> GGUUAAGUUAGGUUUGUGGUUGAAAGUCGAUGCCAGUCGCAGGCAAAACGAUCCACGUAAGUUAAACAAAGUUUUAAUGAGCAUGGUGCGGCUUAGAAGUAAGUCCUGCCGCUUUAGGCGAGAGUAUUAGUAGUGAGAGGGUAAUUCCGGGUAGCGAAACUUCCAGCAGGCGAGUGUGGGGUCAAAGACCAGGUCAACUAACUUA

Here we report three-dimensional structures of three large ornate bacterial RNAs using cryo-electron microscopy (cryo-EM). GOLLD (Giant, Ornate, Lake- and Lactobacillales-Derived), ROOL (Rumen-Originating, Ornate, Large) and OLE (Ornate Large Extremophilic) RNAs form homo-oligomeric complexes whose stoichiometries are retained at lower concentrations than measured in cells. Unexpectedly, the three structures are stabilized not by proteins but by other copies of the same RNA molecule in ornate quaternary assemblies with many intermolecular bridges, a phenomenon that has not previously been observed for natural RNA molecules. Extensive intramolecular and intermolecular A-minor interactions, kissing loops, an unusual A–A helix and other interactions stabilize the three complexes.

First, concomitant with the same set of cryo-EM studies presented above, we resolved a 2.9 Å resolution map of another large RNA molecule, the raiA motif from C. acetobutylicum, as a pure monomer, refuting the possibility that any large RNA would form a multimer in our experimental conditions.> GPGSEFVRRVKTIYDCQADNDDELTFIEGEVIIVTGEEDQEWWIGHIEGQ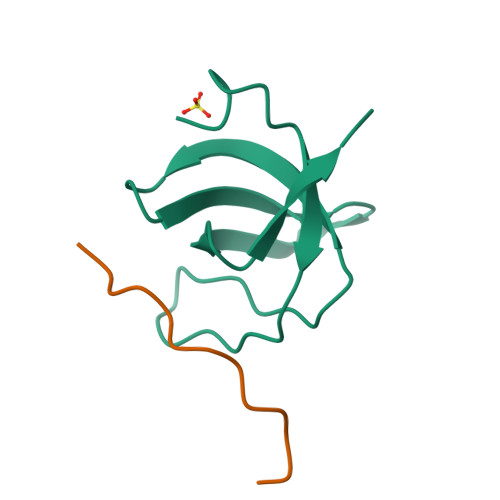PERKGVFPVSFVHILSD;> GPGSEPPPKPPRS>[2x]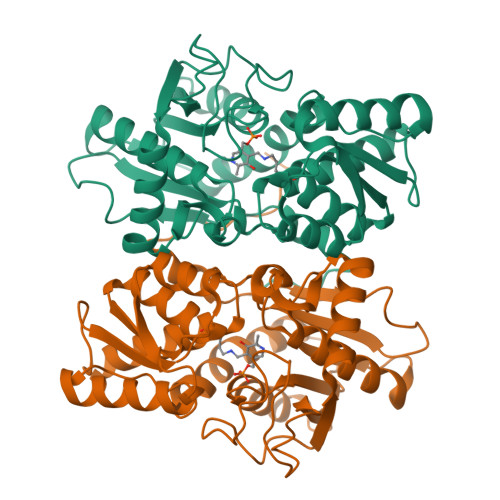MGHHHHHHMAQKPVDNITQIIGGTPVVKLRNVVDDNAADVYVKLEYQNPGGSVKDRIALAMIEKAEREGKIKPGDTIVEPTSGNTGIGLAFVCAAKGYKAVFTMPETMSQERRNLLKAYGAELVLTPGSEAMKGAIKKAKELKEEHGYFEPQQFENPANPEVHELTTGPELLQQFEGKTIDAFLAGVGTGGTLSGVGKVLKKEYPNIEIVAIEPEASPVLSGGEPGPHKLQGLGAGFIPGTLNTEIYDSIIKVGNDTAMEMSRRVAKEEGILAGISSGAAIYAAIQKAKELGKGKTVVTVLPSNGERYLSTPLYSFDD>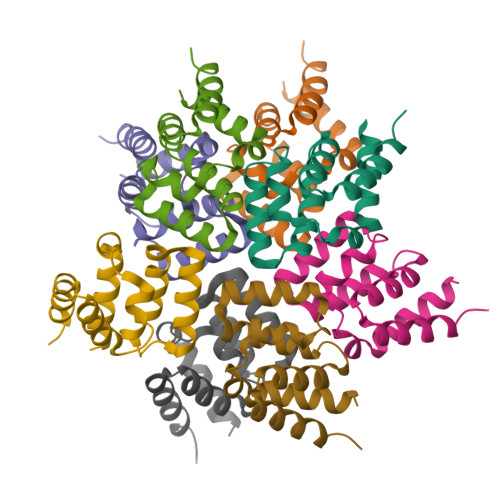[8x]MAFAEDKTYKYICRNFSNFCNVDVVEILPYLPCLTARDQDRLRATCTLSGNRDTLWHLFNTLQRRPGWVEYFIAALRGCELVDLADEVASVYQSYQP> MSSTPEKQTDPKAKANSIINAIPGNNILTKTGVLGTSAAAVIYAISNELYVINDESILLLTFLGFTGLVAKYLAPAYKDFADARMKKVSDVLNASRNKHVEAVKDRIDSVSQLQNVAETTKVLFDVSKETV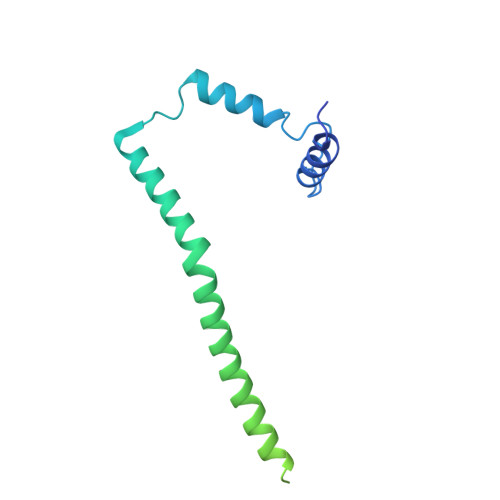ELESEAFELKQKVELAHEAKAVLDSWVRYEASLRQLEQRQLAKSVISRVQSELGNPKFQEKVLQQSISEIEQLLSKLK> TFISRFAPDQPRKGADILVEALERQGVETVFAYPGGASMEIHQALTRSSSIRNVLPRHEQGGVFAAEGYARSSGKPGICIATSGPGATNLVSGLADALLDSVPLVAITGQVPRRMIGTDAFQETPIVEVTRSITKHNYLVMDVEDIPRIIEEAFFLATSGRPGPVLVDVPKDIQQQLAIPNWEQAMRLPGYMSRMPKPPEDSHLEQIVRLISESKKPVLYVGGGCLNSSDELGRFVELTGIPVASTLMGLGSYPEDDELSLHMLGMHGTVYANYAVEHSDLLLAFGVRFDDRVTGKLEAFASRAKIVHIDIDSAEIGKNKTPHVSVCGDVKLALQGMNKVLENRAEELKLDFGVWRNELNVQKQKFPLSFKTFGEAIPPQYAIKVLDELTDGKAIISTGVGQHQMWAAQFYNYKKPRQWLSSGGLGAMGFGLPAAIGASVANPDAI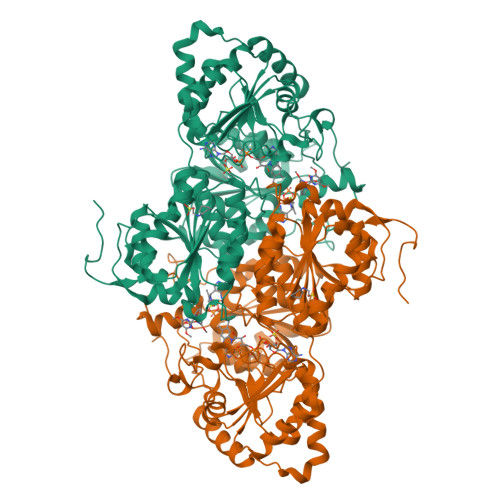VVDIDGDGSFIMNVQELATIRVENLPVKVLLLNNQHLGMVMQLEDRFYKANRAHTFLGDPAQEDEIFPNMLLFAAACGIPAARVTKKADLREAIQTMLDTPGPYLLDVICPHQEHVLPMIPSGGTFNDVITEGDGRLEHHHHHH> SLPENAPNAVSNPQQFITPATALSAEEYNVHEALGETEELELDEFPVLVFKGNVPVDSVTSIPLDLATIYDFAWDGEQNAISQKFQRFAHLIPKSAGGFGPVIGNYTITANLPTGVAGRILHNCLPGDCVDLAVSRIFGLKSLLGVAGTAVSAIGGPLLNGLVNTAAPILSGAAHAIGGNVVGGLADAVIDIGSNLLTPKEKEQPSANSSAISGDIPISRFVEMLKYVKENYQDNPVFPTLLVEPQNFISNAMTALKTIPIEVFANMRNVKVERNLFDRTVVPTVKEATLADIVIPNHMYGYILRDFLQNKRAFQSGTKQNVYFQQFLTVLSQRNIRTHITLNDITSCSIDSESIANKIERVKHYLSTNSSGETTEEFSRTDTGLLPITTRKIVLGESKRRTERYVAETVFPSVRQ;> ADNEVTAEGGKLVQELVYDHSAIPVAPVVETQAEQPEVPVSLVATRKNDTGHLATKWYDFAKISLSNPANMNWTTLTIDPYNNVTLSRDGESMVLPWRRNVWTTGSKSIGYIRTMVAQINIPRPPQISGVLEVKDSINNSSISLVEFGGKVEIPIIPKVMNGLATTASLPRHRLNPWMRTAESKVELQYRIIAFNRTSDIADLNVSVLLRPGDSQFQLPMKPDNNVDTRHFELVEALMYHYDSLRIRGEEQ;> MQNPTQTMHIYDMPLRVIAGLSTLAKTTEEDDNTSTGIVVSEVGEPQVVNHPAWIDPFVAYQLRAPRKNITPDFIFGRADIGNAFSAFLPRRFSAPAVGTRLVVDPVFTYQQRTVLGLYNYFHADFYYIVHVPAPLGTGIYLKIY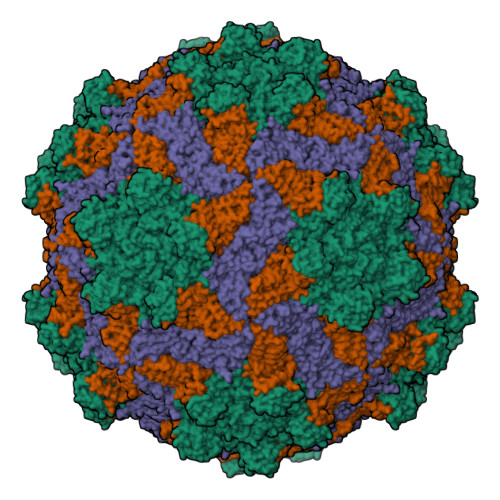APEFDTTTVTRGIRFKPSASPTIALSVPWSNDLSTVETSVGRVGQSGGSIVIETIEDNSNETVNTPLSITVWCCMANIKATGYRHADTSAYNEKGMNFIPVPVPKPPVPPTKPITGEEQ> MTAIGIKTKDGVVLAAERRLSYGDFVLSKSARKVFKLGRFGIAGAGIVGDIQTLTRIMNVEIKYYEMYNSRKISARAAAKLLSVILYQNKVLPYISELLFGGVDEDGPKLFILDPIGSLIEDSYAAVGSGARVAIGVLEAEYNESLTSEA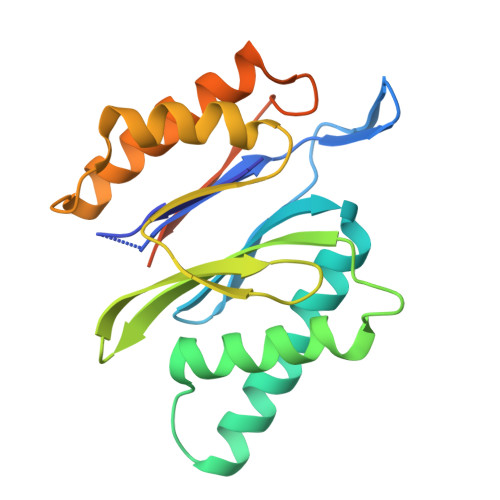AKELAIKSMKSAVERDVMSGDGIDILIINKNNIYEDFIKILEHHHHHH>MSKATYKERAATHPSPVAAKLFNIMHEKQTNLCASLDVRTTKELLELVEALGPKICLLKTH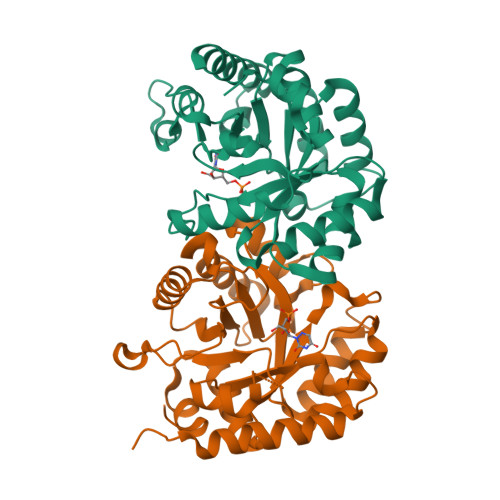VDILTDFSMEGTVKPLKALSAKYNFLLFENRKFADIGNTVKLQYSAGVYRIAEWADITNAHGVVGPGIVSGLKQAAEEVTKEPRGLLMLAELSCKGSLATGEYTKGTVDIAKSDKDFVIGFIAQRDMGGRDEGYDWLIMTPGVGLDDKGDALGQQYRTVDDVVSTGSDIIIVGRGLFAKGRDAKVEGERYRKAGWEAYLRRCGQQN[4x]Crucially, for every round of cap-dependent translation initiation, eIF2 requires GDP-to-GTP exchange, catalyzed by its dedicated guanine nucleotide exchange factor (GEF), eIF2B. Molecularly, eIF2B is a large, heterodecameric complex composed of two copies each of an α, β, γ, δ, and ε subunit. The decameric holoenzyme is built from two eIF2Bβγδε tetramers and one eIF2Bα2 dimer. However, we and others recently discovered that binding of the inhibitor eIF2-P to a distinct binding site — located on the face of the eIF2B complex opposite of the substrate-binding site — allosterically switches eIF2B from its active ‘A-State’ (which can readily engage eIF2 and catalyze nucleotide exchange) to an inhibited ‘I-State’.

Here, we show that a single engineered H to D mutation in eIF2Bβ alters the conformation of the eIF2B decamer, resulting in altered dissociation kinetics of substrate eIF2, a ~ three fold reduction of intrinsic enzymatic activity, and resistance to ISRIB rescue. After 2D and 3D classification, we generated a single consensus structure of the βH160D decamer at 2.8 Å resolution with most side chains clearly resolved. In the WT decamer, βH160 forms a π–π stacking interaction with δ’F452, which is lost in the βH160D eIF2B decamer and leads to the retraction of the short loop bearing this residue. In the βH160D decamer, β’R228 repositions itself within the network of three negative charges (βE163, βD160, and δ’D450) and one aromatic amino acid (δ’F452) to reach a new stable state locally. The loop movement caused by the mutation propagates across the entire tetramer, resulting in the rocking motion observed in Figure 4B. Comparing the βH160D decamer to A-State (eIF2-bound eIF2B) and I-State (eIF2α-P-bound eIF2B) structures, we noticed that its ISRIB binding pocket was 3.3 Å wider in its long dimension than that of the A-State, again reminiscent of the I-State. The widening of the binding pocket can explain why ISRIB fails to assemble βH160D tetramers into octamers or affect GEF activity. An overlay of the βH160D decamer structure with the eIF2B-eIF2 complex structure revealed that the substrate eIF2α binding pocket was widened by 2.9 Å. As established before, a similar pocket widening is observed in the I-State structure of eIF2B (2.6 Å induced by eIF2α-P binding). This widening is predicted to prevent eIF2 from properly engaging the fourth binding site on eIF2Bδ’ and hence turns the decameric eIF2B into conjoined tetramers such that only three of the four eIF2-eIF2B binding interfaces remain readily accessible to eIF2 binding. The βH160D decamer rather represents a continuous distribution of conformations with a more restricted range of motion compared to the WT decamer, and for which the average converges to an I-State like model.

>[2x]MAAPVVAPPGVVVSRANKRSGAGPGGSGGGGARGAEEEPPPPLQAVLVADSFDRRFFPISKDQPRVLLPLANVALIDYTLEFLTATGVQETFVFCCWKAAQIKEHLLKSKWCRPTSLNVVRIITSELYRSLGDVLRDVDAKALVRSDFLLVYGDVISNINITRALEEHRLRRKLEKNVSVMTMIFKESSPSHPTRCHEDNVVVAVDSTTNRVLHFQKTQGLRRFAFPLSLFQGSSDGVEVRYDLLDCHISICSPQVAQLFTDNFDYQTRDDFVRGLLVNEEILGNQIHMHVTAKEYGARVSNLHMYSAVCADVIRRWVYPLTPEANFTDSTTQSCTHSRHNIYRGPEVSLGHGSILEENVLLGSGTVIGSNCFITNSVIGPGCHIGDNVVLDQTYLWQGVRVAAGAQIHQSLLCDNAEVKERVTLKPRSVLTSQVVVGPNITLPEGSVISLHPPDAEEDEDDGEFSDDSGADQEKDKVKMKGYNPAEVGAAGKGYLWKAAGMNMEEEEELQQNLWGLKINMEEESESESEQSMDSEEPDSRGGSPQMDDIKVFQNEVLGTLQRGKEENISCDNLVLEINSLKYAYNISLKEVMQVLSHVVLEFPLQQMDSPLDSSRYCALLLPLLKAWSPVFRNYIKRAADHLEALAAIEDFFLEHEALGISMAKVLMAFYQLEILAEETILSWFSQRDTTDKGQQLRKNQQLQRFIQWLKEAEEESSEDD;>[2x]MPGSAAKGSELSERIESFVETLKRGGGPRSSEEMARETLGLLRQIITDHRWSNAGELMELIRREGRRMTAAQPSETTVGNMVRRVLKIIREEYGRLHGRSDESDQQESLHKLLTSGGLNEDFSFHYAQLQSNIIEAINELLVELEGTMENIAAQALEHIDSNEVIMTIGFSRTVEAFLKEAARKRKFHVIVAECAPFCQGHEMAVNLSKAGIETTVMTDAAIFAVMSRVNKVIIGTKTILANGALRAVTGTHTLALAAKHHSTPLIVCAPMFKLSPQFPNEEDSFHKFVAPEEVLPFTEGDILEKVSVHCPVFDYVPPELITLFISNIGGNAPSYIYRLMSELYHPDDHVL;>[2x]MAAVAVAVREDSGSGMKAELPPGPGAVGREMTKEEKLQLRKEKKQQKKKRKEEKGAEPETGSAVSAAQCQVGPTRELPESGIQLGTPREKVPAGRSKAELRAERRAKQEAERALKQARKGEQGGPPPKASPSTAGETPSGVKRLPEYPQVDDLLLRRLVKKPERQQVPTRKDYGSKVSLFSHLPQYSRQNSLTQFMSIPSSVIHPAMVRLGLQYSQGLVSGSNARCIALLRALQQVIQDYTTPPNEELSRDLVNKLKPYMSFLTQCRPLSASMHNAIKFLNKEITSVGSSKREEEAKSELRAAIDRYVQEKIVLAAQAISRFAYQKISNGDVILVYGCSSLVSRILQEAWTEGRRFRVVVVDSRPWLEGRHTLRSLVHAGVPASYLLIPAASYVLPEVSKVLLGAHALLANGSVMSRVGTAQLALVARAHNVPVLVCCETYKFCERVQTDAFVSNELDDPDDLQCKRGEHVALANWQNHASLRLLNLVYDVTPPELVDLVITELGMIPCSSVPVVLRVKSSDQ;>MDDKELIEYFKSQMKEDPDMASAVAAIRTLLEFLKRDKGETIQGLRANLTSAIETLCGVDSSVAVSSGGELFLRFISLASLEYSDYSKCKKIMIERGELFLRRISLSRNKIADLCHTFIKDGATILTHAYSRVVLRVLEAAVAAKKRFSVYVTESQPDLSGKKMAKALCHLNVPVTVVLDAAVGYIMEKADLVIVGAEGVVENGGIINKIGTNQMAVCAKAQNKPFYVVAESFKFVRLFPLNQQDVPDKFKYKADTLKVAQTGQDLKEEHPWVDYTAPSLITLLFTDLGVLTPSAVSDELIKLYL[2x];>MEFQAVVMAVGGGSRMTDLTSSIPKPLLPVGNKPLIWYPLNLLERVGFEEVIVVTTRDVQKALCAEFKMKMKPDIVCIPDDADMGTADSLRYIYPKLKTDVLVLSCDLITDVALHEVVDLFRAYDASLAMLMRKGQDSIEPVPGQKGKKKAVEQRDFIGVDSTGKRLLFMANEADLDEELVIKGSILQKHPRIRFHTGLVDAHLYCLKKYIVDFLMENGSITSIRSELIPYLVRKQFSSASSQQGQEEKEEDLKKKELKSLDIYSFIKEANTLNLAPYDACWNACRGDRWEDLSRSQVRCYVHIMKEGLCSRVSTLGLYMEANRQVPKLLSALCPEEPPVHSSAQIVSKHLVGVDSLIGPETQIGEKSSIKRSVIGSSCLIKDRVTITNCLLMNSVTVEEGSNIQGSVICNNAVIEKGADIKDCLIGSGQRIEAKAKRVNEVIVGNDQLMEI[2x]> GIEETIDTVITNALQLSQPKPQKQPTAQSTPLTSGVNSQEVPALTAVETGASGQAVPSDVIETRHVVNYKTRSESTLESFFGRSACVTILEVENFNATTDADRKKQFTTWAITYTDTVQLRRKLEFFTYSRFDLEMTFVITERYYASNTGHARNQVYQLMYIPPGAPRPTAWDDYTWQSSSNPSVFYTYGSAPPRMSIPYVGIANAYSHFYDGFARVPLKDETVDSGDTYYGLVTINDFGTLAVRVVNEYNPARITSKIRVYMKPKHVRCW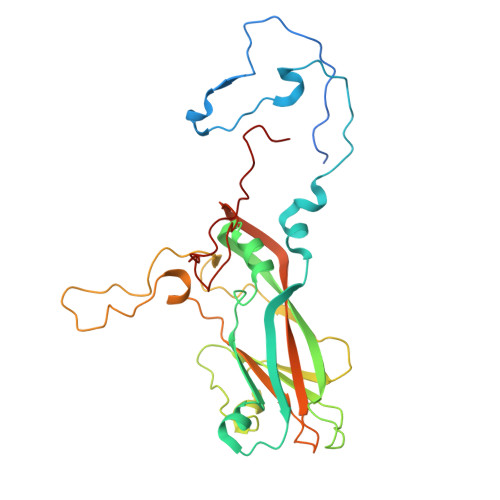CPRPPRAVPYRGEGVDFKQDSITPLTAVENINTF>[13x]MPLVYTPAVRGGANPASGSYLLDPQYVNSGVDILQATYGYNINGTANADQLLQRDAILAILEYALKDTAFVNAIQAVAAGSGVTTPASFVSACVTKLTA;>MAKLNLAVLNNVFSELLTQEINRSATFLGLLSKYPERKSNIQWGVGMGGTTATGVAITGSAPAASMDATLPAQLPISA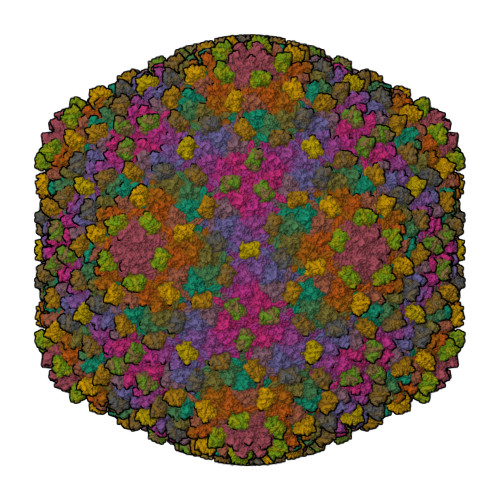ASVQSTFTLNLKEIEESKEQVTNEELRNLLEAQMRNAVEEIATTLNKKLYDGSGAIADGGLIGLSIAASGQDYAGISSATYPLWNVSEVDAWDANATGTDKRQALKTDFMLELDRKIRYRPGAYDLILTTPKVVEQYKKVFEANRSYQIMTFDGQRVPLIDLGFNVAGYMGRPIIDDVFCSRTRTAAESAITTALGTAVDEGVMYFLKKDDLRFYSTPVVGAFSANGVYTLMRQLAQTSLYVDNFVVGCIPQLQLTTRKNVGVIKNIKVG[13x]> DQAQG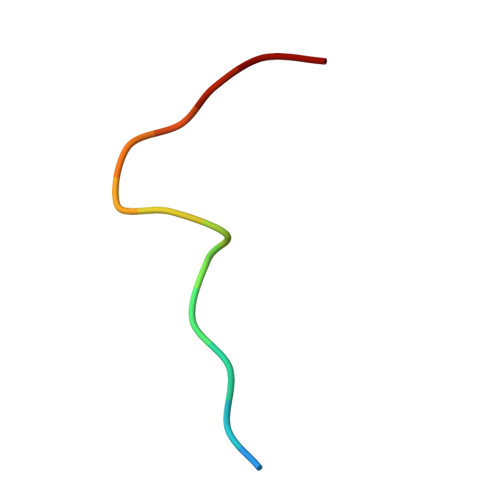PPYPTYIPP N-OMEGA-HYDROXY-L-ARGININE 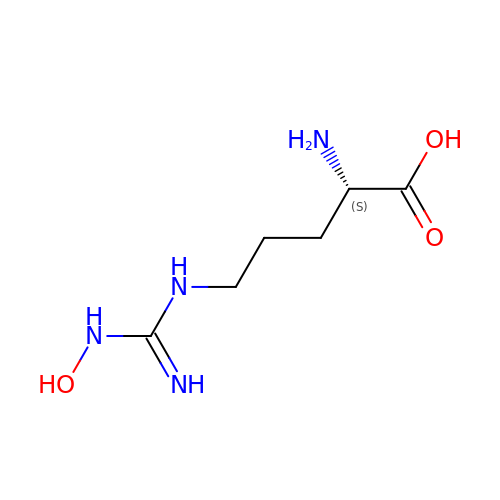| C6 H14 N4 O3 | FQWRAVYMZULPNK-BYPYZUCNSA-N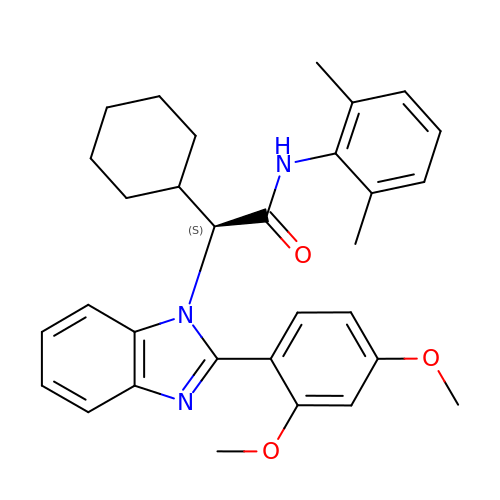(2S)-2-cyclohexyl-2-[2-(2,4-dimethoxyphenyl)-1H-benzimidazol-1-yl]-N-(2,6-dimethylphenyl)acetamide | C31 H35 N3 O3 | AZPPBUOGTWKZCA-LJAQVGFWSA-N> MRGSHHHHHHGSVEYTPW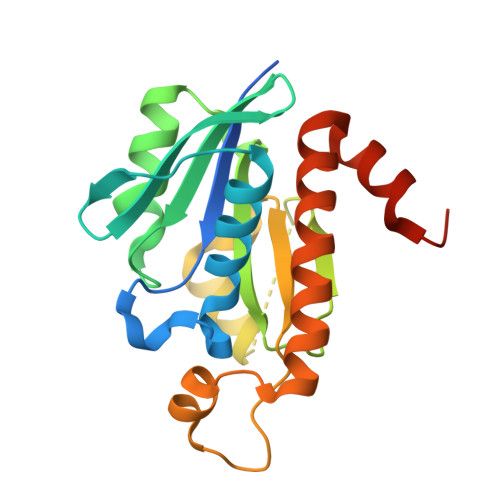LIAGLGNPGNKYYGTRHNVGFEMVDRIAAEEGITMNTEQSKSLLGIGSIGEVPVLVVKPQSYMNYSGEAIGPLAAYYQVPLRHILLIYDDTSLPNGVLRLQKKGGHGRHNGLQNVIEHLDGRREFPRLSIGIGSPPGKMDPRAFLLQKFSSEERVQIDTALEQGVDAVRTLVLKGFSGSTERFNLVQKYKFHRV> MGSSHHHHHHSSGENLYFQHMPFAARLNTPMGPGRTVVVKGEVNANAKSFNVDLLAGKSKDIALHLNPRLNIKAFVRNSFLQE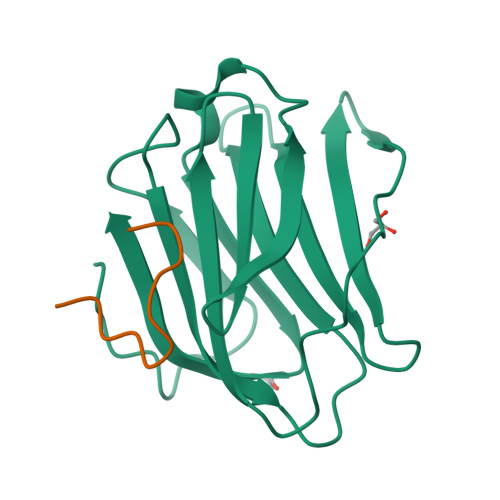SWGEEERNITSFPFSPGMYFEMIIYCDVREFKVAVNGVHSLEYKHRFKELSSIDTLEINGDIHLLEVRSW;> ARQNPGLAYGNPYS>[2x]MGRILFLTTFMSKGNKVVRYLESLHHEVVICQEKVHAQSANLQEIDWIVSYAYGYILDKEIVSRFRGRIINLHPSLLPWNKGRDPVFWSVWDETPKGV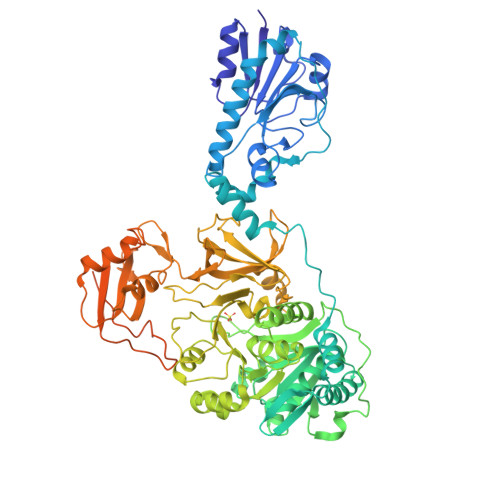TIHLIDEHVDTGDILVQEEIAFADEDTLLDCYNKANQAIEELFIREWENIVHGRIAPYRQTAGGTLHFKADRDFYKNLNMTTVRELLALKRLCAEPKRGEKPIDKTFHQLFEQQVEMTPDHVAVVDRGQSLTYKQLNERANQLAHHLRGKGVKPDDQVAIMLDKSLDMIVSILAVMKAGGAYVPIDPDYPGERIAYMLADSSAAILLTNALHEEKANGACDIIDVHDPDSYSENTNNLPHVNRPDDLVYVMYTSGSTGLAKGVMIEHHNLVNFCEWYRPYFGVTPADKALVYSSFSFDGSALDIFTHLLAGAALHIVPSERKYDLDALNDYCNQEGITISYLPTGAAEQFMQMDNQSFRVVITGGDVLKKIERNGTYKLYNGYGPTECTIMVTMFEVDKPYANIPIGKPIDRTRILILDEALALQPIGVAGELFIVGEGLGRGYLNRPELTAEKFIVHPQTGERMYRTGDRARFLPDGNIEFLGRLDNLVKIRGYRIEPGEIEPFLMNHPLIELTTVLAKEQADGRKYLVGYYVAPEEIPHGELREWLGNDLPDYMIPTYFVHMKAFPLTANGKVDRRALPDVQADAELLGEDYVAPTDELEQQLAQVWSHVLGIPQMGIDDHFLERGGDSIKVMQLIHQLKNIGLSLRYDQLFTHPTIRQLKRLLTEQAAAENLYFQ> AISIKTPEDIEKMRVAGRLAAEVLEMIEPYVKPGVSTGELDRICNDYIVNEQHAVSACLGYHGYPKSVCISINEVVCHGIP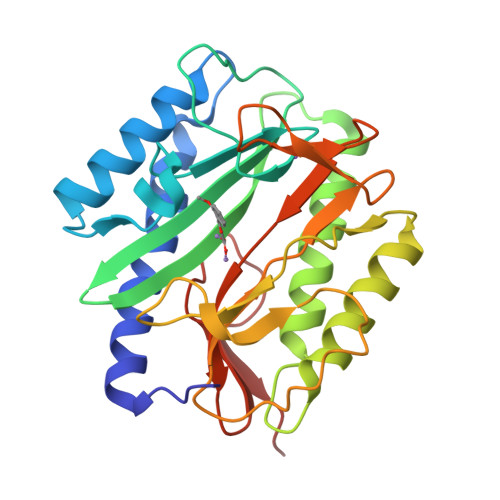DDAKLLKDGDIVNIDVTVIKDGFHGDTSKMFIVGKPTIMGERLCRITQESLYLALRMVKPGINLREIGAAIQKFVEAEGFSVVREYCGHGIGRGFHEEPQVLHYDSRETNVVLKPGMTFTIEPMVNAGKKEIRTMKDGWTVKTKDRSLSAQYEHTIVVTDNGCEILTLRKDDTIPAIISHDE5-{[(3S)-3-(prop-1-yn-1-yl)-4-{4-[S-(trifluoromethyl)sulfonimidoyl]phenyl}piperazin-1-yl]sulfonyl}pyridin-2-amine | C19 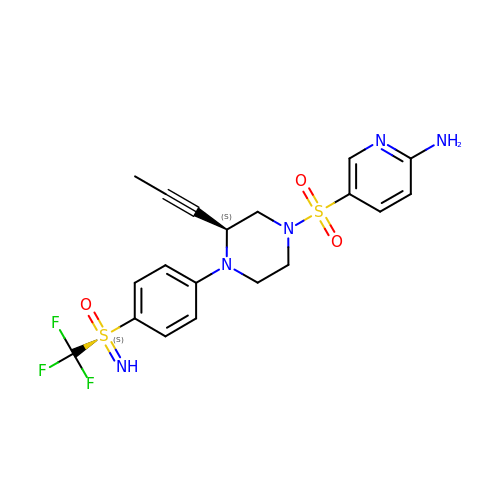H20 F3 N5 O3 S2 | ULWPZVFGWXVNBJ-IWAYBZMOSA-N> MGHHHHHHMAGEVVKSQKKRIRLGKVVPSSIRIVLDCAFDDLMNDKEINSLCQQVTRCHSANRTALHPVELFATNFGGRLKTRQDFVL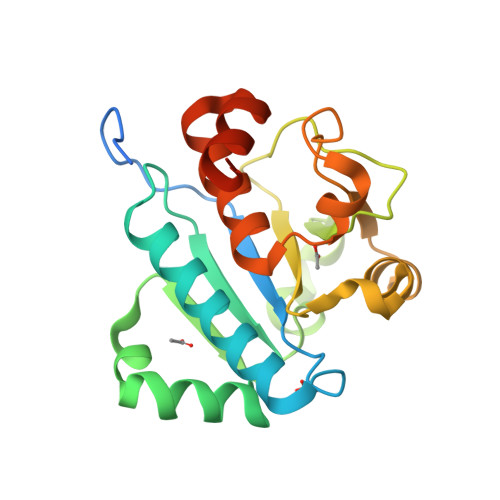KGQQNNWKRYNPTTKSYLEEFESQKEKLVYLSADSDNTITELDEDKIYIIGAIVDKNRYKNLCQNKASEQGIKTAKLPIDEYIKITDRKILTVNQVFEILSLWLEYRDWEKAFMEVIPKRKGILLKSDE>SMFIKKIKAKANNNEINVIIEIPMNSGPIKY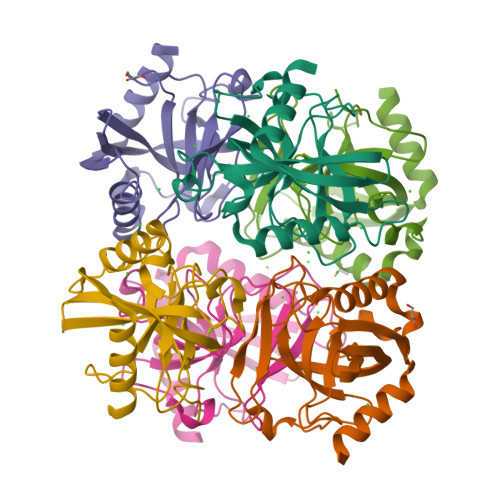EFDKESGALFVDRFMQTTMSYPCNYGFIPDTLSNDGDPVDVLVVAHHPVVPGSVIKCRAIGVLMMEDESGLDEKIIAVPTSKLDITFDHIKELDDLCEMLKKRIVHFFEHYKDLEKGKWVKVTGWGDKVKAETLIKEGIDRN[6x]> KPRVLFSQAQVYELERRFKQQRYLSAPERDQLASVLKLTSTQVKIWFQNRR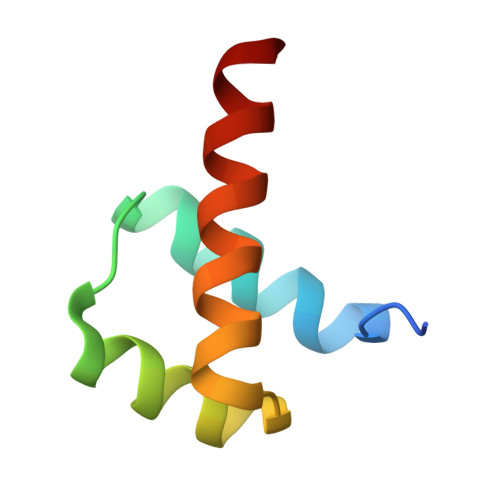YKSKRQ>MKKIPEPFAVTLSLAGLLWSAWALAEDAATKVTDPHFKLAPGYLEPADLPVRLALLGAPPKPGSAALARDEEARRAALALRGSSREKLAATDAELSFPGPAKTFSCALGTQISEKSTPHLYTLMQRTLTDAGGSTYAGKNAYNRTRPFVVHDEGTCRKDMEPLLRTDGSWPSGHSAAGWAWGLVLAEISPARATELMTRGLAYGQSRVICDAHWQSDVDAGRIMGAATVASLHGNPAFLADLAAAKEEVKAAQQAGLKPAEDCAAEGVALGLTQ[4x]

M2‐32 is a non‐specific acid phosphatase with a rare ability to function across a broad pH range (3.5–8.5). Analysis using SWISS‐PROT Prf Profiles classifies it as a class A acid phosphatase (Z‐score: 78.97), sharing 50%–60% sequence similarity with enzymes such as PhoC and PhoN. Although the monomeric form of M2‐32 has a molecular weight of ~28 kDa, size exclusion chromatography, dynamic light scattering, and sedimentation studies revealed a dimeric form in solution. The mechanism of catalysis of histidine phosphatases involves a nucleophilic attack by a conserved histidine (residue His 174 in M2‐32) to generate a covalent phosphoenzyme intermediate (Ishikawa et al., 2000), followed by hydrolysis to release inorganic phosphate that requires protonation of the leaving group by another His (residue 213 in M2‐32).

The truncated model generated by AF2 enabled the determination of the M2‐32 crystal structure at a resolution of 2.2 Å, derived from a crystal belonging to the P 22 1 2 1 space group. The structure revealed that M2‐32 forms a tetramer, with a Matthews coefficient of 2.5 and a solvent content of 51.4%. In the crystal, the tetramer adopts a dimer‐of‐dimers arrangement (A‐C/B‐D), with a buried area of 1129.5/1137.1 Å2, and a free energy change upon interface formation of −23.5/−22.8 kcal/mol, as determined by the PISA server (Krissinel & Henrick, 2007). Each monomer includes residues 45–271 exhibiting an all‐alpha fold arranged with 14 helices (60%), connected by turns (5%) and coils (35%) regions. The structure is stabilized by two disulfide bridges and belongs to the “acid phosphatase class A” protein fold superfamily (SCOP). The first disulfide bridge forms between Cys105 in helix H4 and Cys263 in helix H14, while the second bridge links Cys156 and Cys210, both residing in the loops regions. M2‐32, however, presents an additional extra bridge on the opposite side to the active site of the enzyme. DSF assays suggest that M2‐32 is a thermotolerant enzyme with an unfolding T m of 47°C and, accordingly, this high stability may be conferred by the presence of two sulfide bridges in the monomer, which contrasts with most acid phosphatases that have only one disulfide bridge. Docking studies with adenosine monophosphates, combined with site‐directed mutagenesis, identified His174, Arg207, His213, Asp217 as critical catalytic residues, and Tyr136 and Ser172 probably involved in substrate recognition. Mutations at these positions resulted in over 90% loss of enzymatic activity, highlighting their functional significance.>MPRRDRNMDSAPCMWMRGGTSKGGYFLRADLPADTAARDAFLLAVMGSPDPRQIDGMGGADPLTSKVAVVSKSERPGIDVDYLFLQVFVDQAIVTDAQNCGNILAGVGPFAIERGLVAASGDETRVAIFMENTGQVAVATVRTPGGSVTYAGDAAIDGVPGTHAPIPTEFRDTAGSSCGALLPSGNAVDVVNGLPVTLIDNGMPCVVMKAADVGITGYEDRDSLDANAELKAKIEAIRLAVGELMNLGDVTEKSVPKMMLVAPPRDGGAVCVRSFIPHRAHATIGVLGAVSVATACLIPGSPAAEVAVVPEGARKTLSIEHPTGEMSCVLEVDDAGNVVSAALLRTARKLMDGVVFVLEHHHHH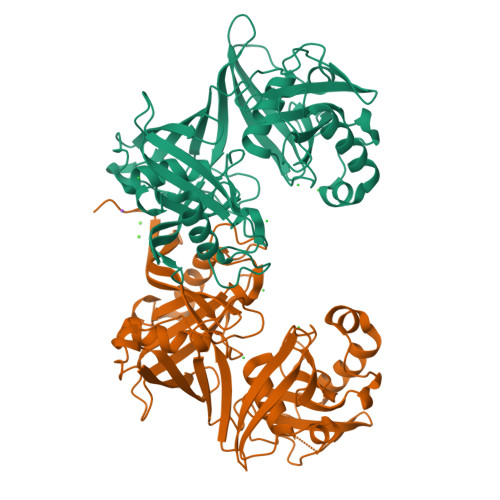H[2x]>MQLWDINDHPYLNIKGRFQRDEN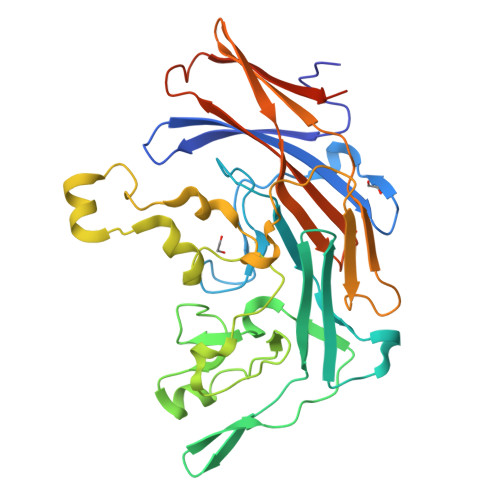GDEVWVVSAKRMWSLTQNEWLSADEVEIFDDPLYAGEPGFSAMIHDHEFAIHKHCTDVVVSGKARAYAKRPVEQMECRLLLDGHIDKTLVIHGQRDWIEHGGSITVSNPQSFIDCDIDYSHAIGGEDERNRIGGGVASSNKVLLTQRVPSVFYPKEDWDATSKKVRVAGFGPIPPFFKQRYQLAGTFDDNWLENRRPLLPVDFDRRYYQSAPLDQQCKGYLQGGERLMLSGFSHDDIFSFRLPREKYRASADFGDDQEFKDLELYTVFVDTEKGVVSLTYSAAFACQEKEHLLKSTSIQAVVENTNERGLNNEKLEHHHHHH[2x]> QEEEYSG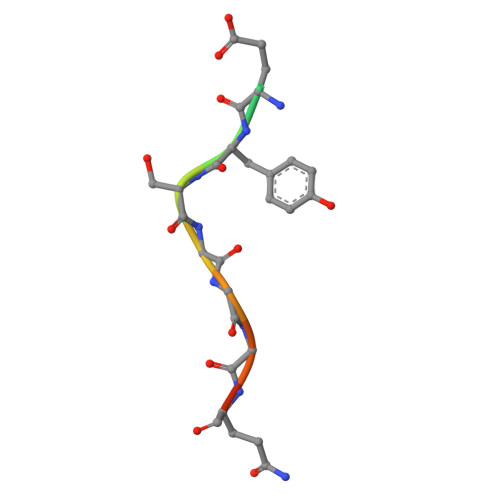GGQGG>GMEFLMKISHLDHLVLTVADIPTT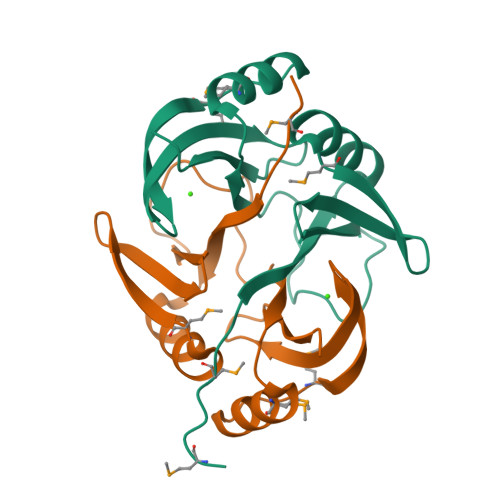TNFYEKVLGMKAVSFGAGRIALEFGHQKINLHQLGNEFEPKAQNVRVGSADLCFITDTVLSDAMKHVEDQGVTIMEGPVKRTGAQGAITSFYFRDPDGNLIEVSTYSNT[2x]>[2x]GSDYENDDECWSVLEGFRVTLTSVIDPSR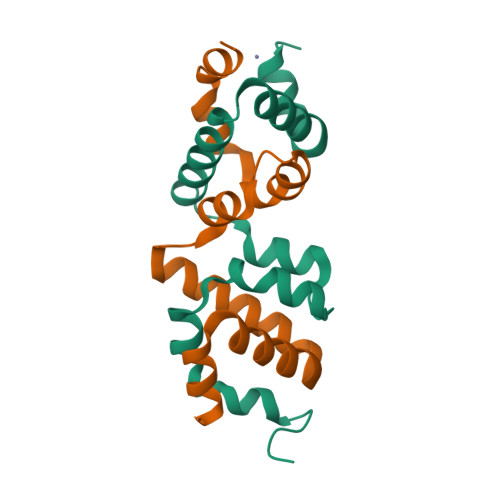ITPYLRQCKVLNPDDEEQVLSDPNLVIRKRKVGVLLDILQRTGHKGYVAFLESLELYYPQLYKKVTGK>[2x]MAPITAYSQQT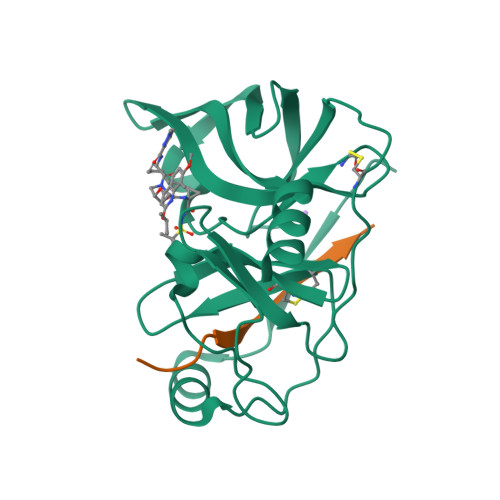RGLLGCIITSLTGRDKNQVDGEVQVLSTATQSFLATCVNGVCWTVYHGAGSKTLAGPKGPITQMYTNVDQDLVGWPAPPGARSMTPCTCGSSDLYLVTRHADVIPVRRRGDSRGSLLSPRPVSYLKGSSGGPLLCPSGHVVGIFKAAVCTRGVAKAVDFIPVESMETTMRASKKKK;>[2x]KKGSVVIVGRIILSGRK(3S)-3-(2-fluorophenyl)-N-((2-oxo-2,3-dihydro-1H-benzo[d]imidazol-5-yl)methyl)butanamide) | C18 H18 F N3 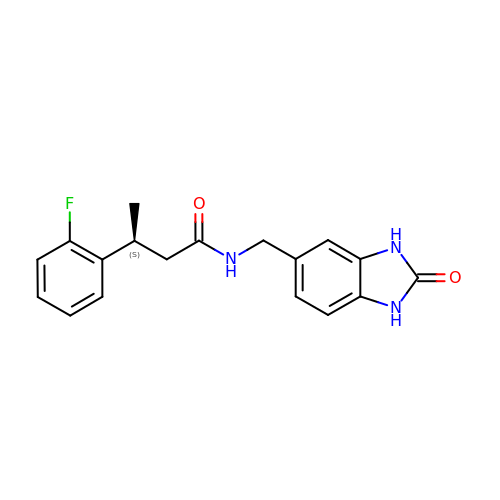O2 | JYQMTEASQYBLAO-NSHDSACASA-N> SPNSQYLKTRILDIYTPEQRAGIEKSEDWRQFSRRMDTHFPKLMNELDSVYGNNEALLPMLEMLLAQAWQSYSQRNSSLKDIDIARENNPDWILSNKQVGGVCYVDLFAGDLKGLKDKIPYFQELGLTYL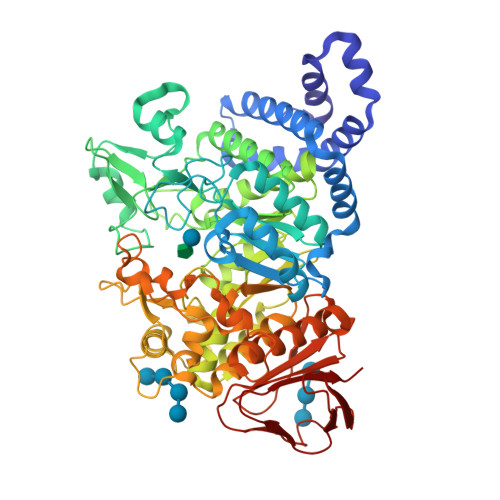YLMPLFKCPEGKSDGGYAVSSYRDVNPALGTIGDLREVIAALHEAGISAVVDFIFNHTSNEHEWAQRCAAGDPLFDNFYYIFPDRRMPDQYDRTLREIFPDQHPGGFSQLEDGRWVWTTFNSFQWDLNYSNPWVFRAMAGEMLFLANLGVDILRMDAVAFIWKQMGTSCENLPQAHALIRAFNAVMRIAAPAVFFKSQAIVHPDQVVQYIGQDECQIGYNPLQMALLWNTLATREVNLLHQALTYRHNLPEHTAWVNYVRSHDDIGWTFADEDAAYLGISGYDHRQFLNRFFVNRFDGSFARGVPFQYNPSTGDCRVSGTAAALVGLAQDDPHAVDRIKLLYSIALSTGGLPLIYLGDEVGTLNDDDWSQDSNKSDDSRWAHRPRYNEALYAQRNDPSTAAGQIYQGLRHMIAVRQSNPRFDGGRLVTFNTNNKHIIGYIRNNALLAFGNFSEYPQTVTAHTLQAMPFKAHDLIGGKTVSLNQDLTLQPYQVMWLEIA> DQRNASYPHCLQFYLQPPSENISLIEFENLAIDRVKLLKSVENLGVSYVKGTEQYQSKLESELRKLKFSYRENLEDEYEPRRRDHISHFILRLAYCQSEELRRWFIQQEMDLLRFRFSILPKDKIQDFLKDSQLQFEAISDEEKTLREQEIVASSPSLSGLKLGFESIYKIPFADALDLFRGRKVYLEDGFAYVPLKDIVAIILNEFR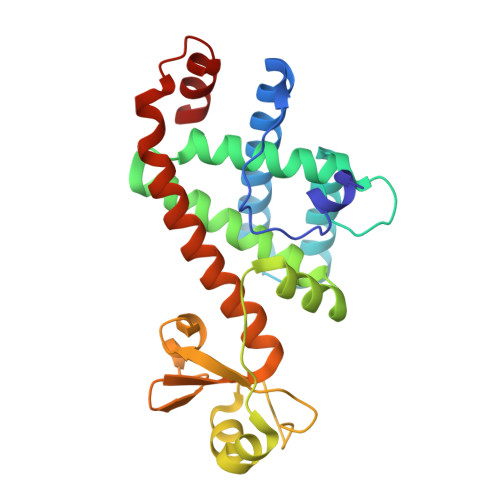AKLSKALALTARSLPAVQSDERLQPLLNHLSHS>[2x]FYNPPTNVVSHVNGDWFLFGDSRSDCNHIGNINPHNYSYMDLNPALCDSGKISSKAGNSIFRSFHFTDFYNYTGEGQQIIFYEGVNFTPYHAFKCNRSGSNDIWMQNKGLFYTQVYKNMAVYRSLTFVNVSYVYNGSAQATAFCKSGSLVLNNPAYIAPQANSGIITKVEADFYLSGCDEY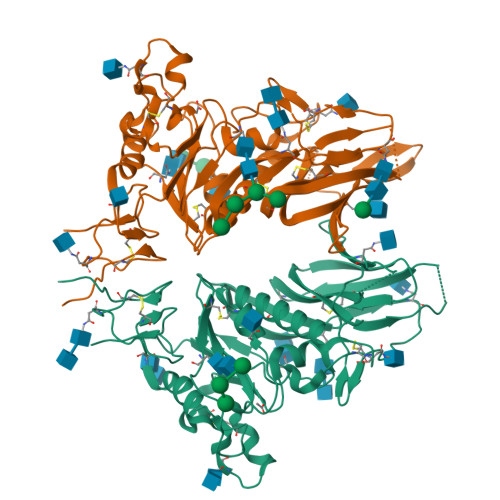IVPLCIFNGKFLSNTKYYDHSQYYFNKDTGVIYGLNSTETITTGFDLNCHYLVLPSGNYLAISNELLLTVPTKAICFNKRKDFTPVQVVDSRWNNARQSDNMTAVACQPPYCYFRNSTTNYVGVYDINHGDAGFTSILSGLLYNSSCFSQQGVFRYDNISSVWPLYPYGRCPTAADINIPDLPICVYDSDPLVPR> EAEFQYFGSYYCQPGRDVIVHLFEWKWTDIERECQWLADHNYCGVQVSPPNEHRIVTDPPYPWWQRYQ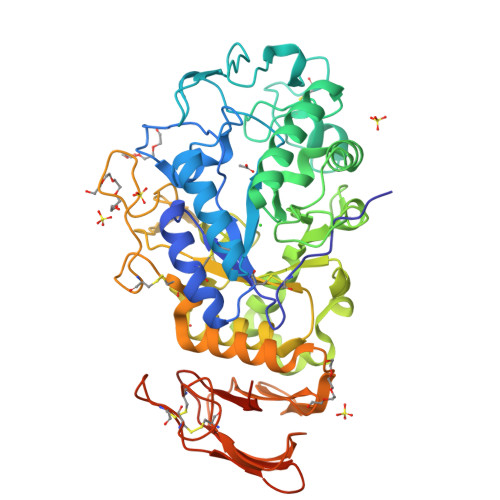PVSYTMNSRSGSETQFRNMVTTCNNLGVYIYVDGVLNHMTGGGSGTGSDGNSFDGDSLQYPGVPYGPNDFHGSDDCSTSDGEIHDYNNPTEVRNCRLSGLRDLDGSANYVRDVEAEFANRLIGWGVAGFRLDACKHMWPGDLEAILGRLNQLNTQWFPAGRNAYIYQEVIDLGGEAVKATEYTYLGRVTEFKHGQNLGNVVRKNNGQRLANLVNFGEGWGQLSGFDALVFIDNHDNQRGHGAGGFGTILTFFEANMYKIATAFELAWDYGHVRLMSSYNWPRNIVNGVDTNDWVGPPTNGGGDTKDVECFNGEWICEHRWREMYNMVRFHNVAIGNPVSNWWDNGFQAIAFGRGNRGFIFINNEDFAITQTLQTGLPGGEYCDVISCDNNRPPCGNSGGACRATVIVNGDGTATFDVPNGENPMIAIHVFLEQKLISEEDLNSAVDHHHHHH>EQARPADDALAALGAQLFVDPALSRNATQSCATCHDPARAFTDPREGKAGLAVSVGDDGQSHGDRNTPTLGYAALVPAFHRDANGKYKGGQFWDGRADDLKQQAGQPMLNPVEMAMPDRAAVAARLRDDPAYRTGFEALFGKGVLDDPERAFDAAAEALAAYQATGEFSPFDSKYDRVMRGEEKFTPLEEFGYTVFITENCRLCHMQRKQGVAERETFTNFEYHNIGLPVNETAREASGLGADHVDHGLLARPGIEDPAQSGRFKVPSLRNVAVTGPYMHNGVFTDLRTAILFYNKYTSRRPEAKINPETGAPWGEPEVARNLSLAELQSGLMLDDGRVDALVAFLETLTDRRYEPLLEESRAAQKDHHHHHH[2x];>[2x]ADAPAGTDPRAKWVPQDNDIQACDYWRHCSIDGNICDCSGGSLTNCPPGTKLATASWVASCYNPTDGQSYLIAYRDCCGYNVSGRCPCLNTEGELPVYRPEFANDIIWCFGAEDDAMTYHCTISPIVGKASHHHHHH;>QDAPEAETQAQETQGQAAARAAAADLAAGQDDEPRILEAPAPDARRVYVNDPAHFAAVTQQFVIDGEAGRVIGMIDGGFLPNPVVADDGSFIAHASTVFSRIARGERTDYVEVFDPVTLLPTADIELPDAPRFLVGTYPWMTSLTPDGKTLLFYQFSPAPAVGVVDLEGKAFKRMLDVPDCYHIFPTAPDTFFMHCRDGSLAKVAFGTEGTPEITHTEVFHPEDEFLINHPAYSQKAGRLVWPTYTGKIHQIDLSSGDAKFLPAVEALTEAERADGWRPGGWQQVAYHRALDRIYLLVDQRDE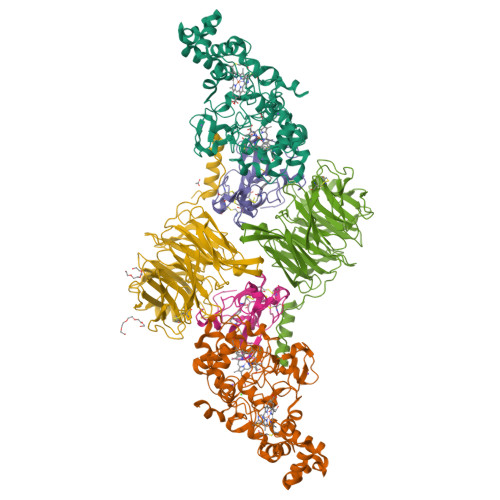WRHKTASRFVVVLDAKTGERLAKFEMGHEIDSINVSQDEKPLLYALSTGDKTLYIHDAESGEELRSVNQLGHGPQVITTADMG[2x]(2S)-HEX-5-ENE-1,2-DIOL 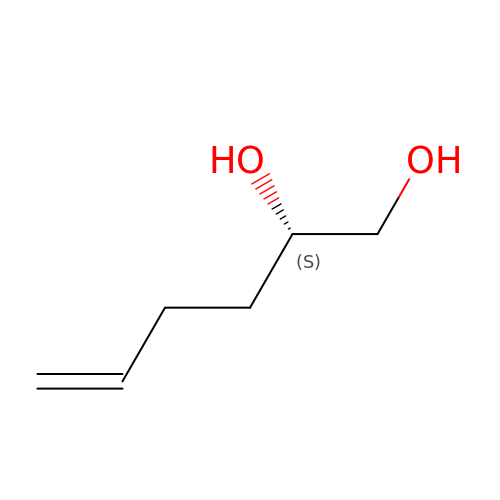| C6 H12 O2 | WGTGQGJDNAGBCC-LURJTMIESA-N>AIETETLVVGAGPGGYVAAIRAAQLGQKVTIVEKGNLGGVCLNVGCIPSKALISASHRYEQAKHSEEMGIKAENVTIDFAKVQEWKASVVKKLTGGVEGLLKGNKVEIVKGEAYFVDANTVRVVNGDSAQTYTFKNAIIATGSRPIELPNFKFSNRILDSTGALNLGEVPKSLVVIGGGYIGIELGTAYANFGTKVTILEGAGEILSGFEKQMAAIIKKRLKKKGVEVVTNALAKGAEEREDGVTVTYEANGETKTIDADYVLVTVGRRPNTDELGLEQIGIKMTNRGLIEVDQQCRTSVPNIFAIGDIVPGPALAHKASYEGKVAAEAIAGHPSAVDYVAIPAVVFSDPECASVGYFEQQAKDEGIDVIAAKFPFAANGRALALNDTDGFLKLVVRKEDGVIIGAQIIGPNASDMIAELGLAIEAGMTAEDIALTIHAHPTLGEIAMEAAEVAL[2x];> IAMPSVRKYAREKGVDIRLVQGTGKNGR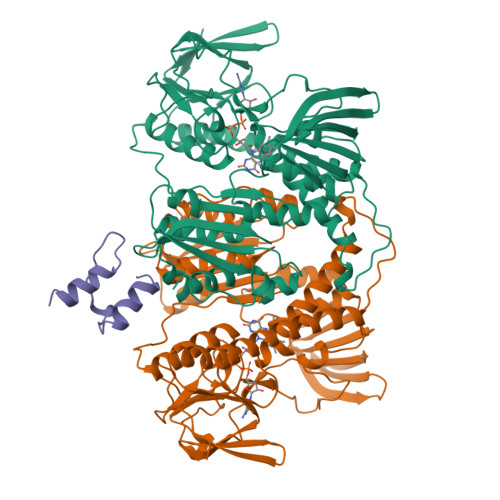VLKEDIDAFLAGG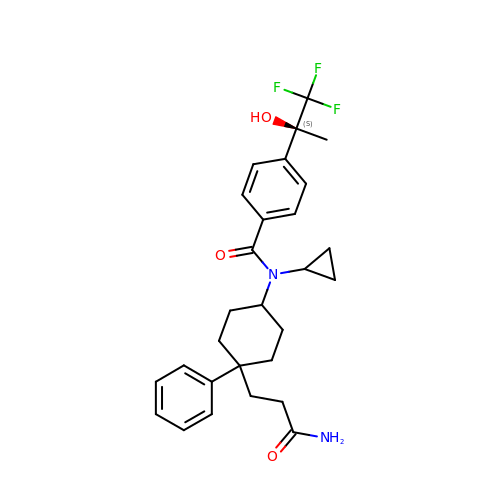N-[trans-4-(3-amino-3-oxopropyl)-4-phenylcyclohexyl]-N-cyclopropyl-4-[(1S)-2,2,2-trifluoro-1-hydroxy-1-methylethyl]benzamide | C28 H33 F3 N2 O3 | GGXWRFSOCBTDDI-YGPDHOBYSA-N Pyridoxal 5’-phosphate phosphatase (PDXP), an enzyme that controls levels of pyridoxal 5’-phosphate (PLP), the co-enzymatically active form of vitamin B6, may represent an alternative therapeutic entry point into vitamin B6-associated pathologies. PDXP is a member of the large family of haloacid dehalogenase (HAD)-type hydrolases. HAD phosphatases are Mg2+-dependent phospho-aspartate transferases that consist of a Rossman-like catalytic core linked to a cap domain. 7,8-DHF binds and reversibly inhibits PDXP with low micromolar affinity and sub-micromolar potency.

We additionally obtained two co-crystal structures of human PDXP with 7,8-DHF: one in a phosphate-containing and one in a phosphate-free form. In contrast to murine PDXP, 7,8-DHF bound to human PDXP with a ratio of two inhibitors per homodimer and well-defined density. Interestingly, the orientation of the inhibitor was markedly affected by the presence or absence of phosphate. In the absence of phosphate, the inhibitor is flipped horizontally, with the hydroxylated chromone substructure of 7,8-DHF now located closest to the Mg2+ ion (compare left and right panels). Inhibitor binding in the absence of phosphate is primarily stabilized by metal coordination and hydrogen bonds, as well as polar and non-polar interactions. The 7-hydroxyl group of 7,8-DHF is involved in an octahedral Mg2+ coordination, albeit with an elongated oxygen-Mg2+ distance of 2.7 Å, leading to the displacement of a water molecule. The 8-hydroxyl group of 7,8-DHF forms a hydrogen bond with Arg239 and His182. The ketone group of the inhibitor participates in a water-bridged hydrogen bond to the carboxyl group of Asp27 and the backbone amine group of Gly33. Interestingly, Glu152 (or Glu148) and Arg62 can form an intramolecular salt bridge that obstructs the active site entrance. This interaction was observed in phosphate-free 7,8-DHF-hPDXP and phosphate-free PLP-hPDXP, as well as in apo-hPDXP and apo-mPDXP.

> MARCERLRGAALRDVLGRAQGVLFDCDGVLWNGERAVPGAPELLERLARAGKAALFVSNNSRRARPELALRFARLGFGGLRAEQLFSSALCAARLLRQRLPGPPDAPGAVFVLGGEGLRAELRAAGLRLAGDPSAGDGAAPRVRAVLVGYDEHFSFAKLREACAHLRDPECLLVATDRDPWHPLSDGSRTPGTGSLAAAVETASGRQALVVGKPSPYMFECITENFSIDPARTLMVGDRLETDILFGHRCGMTTVLTLTGVSRLEEAQAYLAAGQHDLVPHYYVESIADLTEGLED> AREPLTSYLDSQYFGKIYIGTPPQEFTVVFDTGSSDLWVP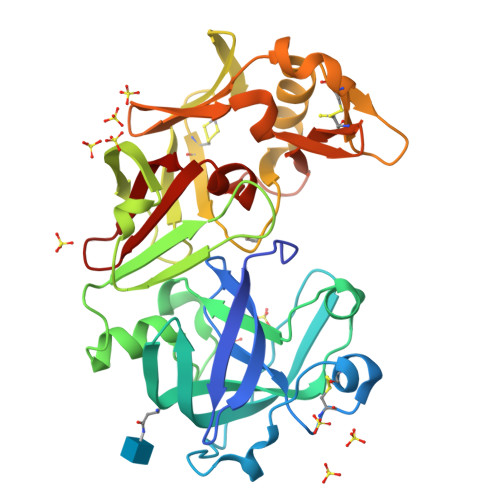SIYCKSNVCKNHHRFDPRKSSTFRNLGKPLSIHYGTGSMEGFLGYDTVTVSNIVDPNQTVGLSTEQPGEVFTYSEFDGILGLAYPSLASEYSVPVFDNMMDRHLVARDLFSVYMDRNGQGSMLTLGAIDPSYYTGSLHWVPVTLQQYWQFTVDSVTINGVAVACVGGCQAILDTGTSVLFGPSSDILKIQMAIGATENRYGEFDVNCGNLRSMPTVVFEINGRDYPLSPSAYTSKDQGFCTSGFQGDNNSELWILGDVFIREYYSVFDRANNRVGLAKAI>MGKSTLKHTRKIQILIDLPTKDEKKEVMDMMYQWRDRCFRAANIIVTHLYVQEMIKDFFYLSEGIKYKLADEKKDEKGILQRSRMNTTYRVVSDRFKGEMPTNILSTLNHGLISSFNKNRVQYWKGERSLPNFKKDMAFPFGLQGISRLVYDEEKKAFCFRLYRVPFKTYLGKDFTDKRMLLERLVKGDVKLCASNIQLNGGKIFWLAVFEIEKEKHSLKPEVIAEASLSLEYPIVVKTGKNRLTIGTKEEFLYRRLAIQAARRRTQVGATYSRSGKGKKRKLKAV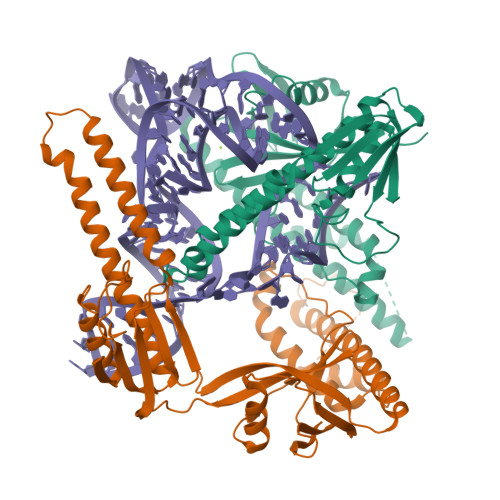DKYHKTESNYVAHRIHVYSRKLIDFCIKHQAGTLILMNQEDKVGIAKEEEFVLRNWSYYELMTKIKYKAEKAGIELIIG[2x]> GPGSDKDCEMKRTTLDSPLGKLELSGCEQGLHEIIFLGKGTSAADAVEVPAPAAVLGGPEPLMQATAWLNAYFHQPEAIEEFPVPALHHPVFQQESFTRQVLWKLLKVVKFGEVISYSHLAALAGNPAATAAVKTALSGNPVPILIPCHRVVQGDLD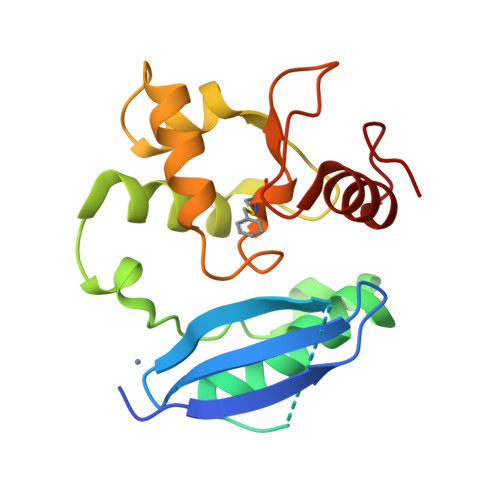VGGYEGGLAVKEWLLAHEGHRLGKR>[3x]MELMMAIGYLGLALVLGSLVAKIAEKLKIPDIPLLLLLGLIIGPFLQIIPSDSAMEIFEYAGPIGLIFILLGGAFTMRISLLKRVIKTVVRLDTITFLITLLISGFIFNMVLNLPYTSPVGYL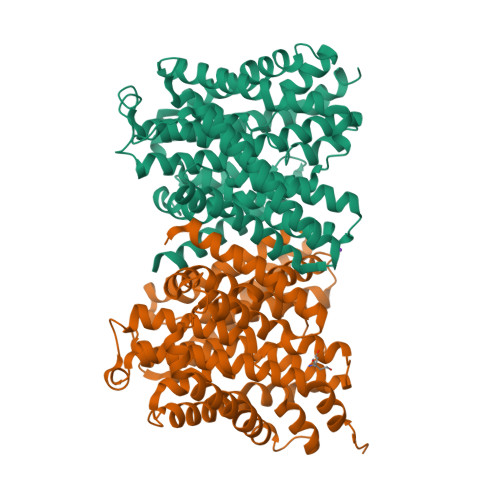FGAITAATDPATLIPVFSRVRTNPEVAITLEAESIFNDPLGIVSTSVILGLFGLFSSSNPLIDLITLAGGAIVVGLLLAKIYEKIIIHCDFHEYVAPLVLGGAMLLLYVGDDLLPSICGYGFSGYMAVAIMGLYLGDALFRADDIDYKYIVSFCDDLSLLARVFIFVFLGACIKLSMLENYFIPGLLVALGSIFLARPLGVFLGLIGSKHSFKEKLYFALEGPRGVVPAALAVTVGIEILKNADKIPASITKYITPTDIAGTIIIGTFMTILLSVILEASWAGMLALKLLGEYKPKYKEESHH;> MELMMAIGYLGLALVLGSLVAKIAEKLKIPDIPLLLLLGLIIGPFLQIIPSDSAMEIFEYAGPIGLIFILLGGAFTMRISLLKRVIKTVVRLDTITFLITLLISGFIFNMVLNLPYTSPVGYLFGAITAATDPATLIPVFSRVRTNPEVAITLEAESIFNDPLGIVSTSVILGLFGLFSSSNPLIDLITLAGGAIVVGLLLAKIYEKIIIHCDFHEYVAPLVLGGAMLLLYVGDDLLPSICGYGFSGYMAVAIMGLYLGDALFRADDIDYKYIVSFCDDLSLLARVFIFVFLGACIKLSMLENYFIPGLLVALGSIFLARPLGVFLGLIGSKHSFKEKLYFALEGPRGVVPAALAVTVGIEILKNAEKIPASITKYITPTDIAGTIIIGTFMTILLSVILEASWAGMLALKLLGEYKPKYKEESHH> MQLRRYAATLSEGDIIVIPSSFPVALKAASDLNMVGIGVNAENNERNFLAGHKEN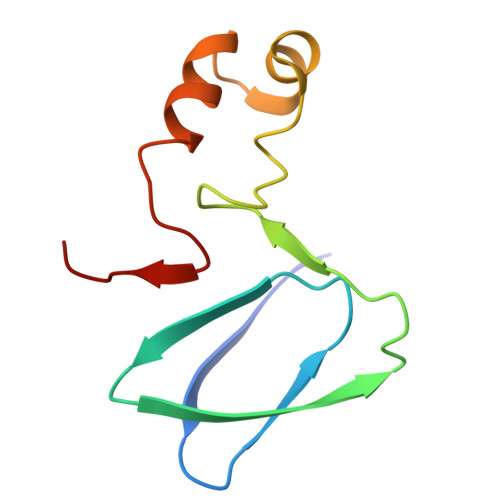VIRQIPRQVSDLTFPGSGEEVEELLENQKESYFVDGQP Here we focus on EndoE, a multi-modular glycoside hydrolase secreted by Enterococcus faecalis, one of the leading causes of healthcare-associated infections. We provide X-ray crystal structures of EndoE, which show an architecture composed of four domains, including GH18 and GH20 glycoside hydrolases connected by two consecutive three α-helical bundles. We determine that the GH20 domain is an exo-β-1,2-N-acetylglucosaminidase, whereas the GH18 domain is an endo-β-1,4-N-acetylglucosaminidase that exclusively processes the central core of complex-type or high-mannose-type N-glycans. Both glycoside hydrolase domains act in a concerted manner to process diverse N-glycans on glycoproteins, including therapeutic IgG antibodies.

EndoE-GH20 crystallized in the P 1 2 1 1 space group with one molecule in the asymmetric unit and diffracted to a maximum resolution of 1.4 Å. The quality of the electron density maps allowed us to trace residues 489–835. The GH20 domain adopts the conserved (β/α)8-barrel topology with an overall size of 55 × 50 × 39 Å. A long and open groove, including a deep pocket, runs parallel to the protein surface and contains the active site. This groove is located at the center of the (β/α)8-barrel and surrounded by the loops connecting β1-α1 (loop 1; residues 499–505, pink), β2-β3 (loop 2; residues 530–541, brown), β5-α4 (loop 3; residues 598–603, orange), β6-α6 (loop 4; residues 660–670, light green), β7-β8 (loop 5; residues 706–724, blue), β8-α7 (loop 6; residues 729–740, green), β9-α8 (loop 7; residues 754–771, light blue), and β10-α9 (loop 8; residues 804–813, red). In a first step, D661 stabilizes the reaction intermediate and orients the acetamido oxygen for nucleophilic attack on the anomeric carbon to form an oxazolium ion intermediate. In addition, E662 acts as an acid protonating the glycosidic bond. Structural comparison of GH20 domain of EndoE with LNBase showed that the conformation and length of loops 1 and 8 in EndoE-GH20 could block the entrance of an extra carbohydrate moiety linked to GlcNAc (-1), confirming the exo-activity of this domain. The GH20 domain of EndoE cannot accommodate bisecting CT N-glycans due to the presence of bulky and hydrophobic residues in loop 7 that block the access of the additional β(1,4)-GlcNAc to the binding site, as in the case of the GH20A domain of StrH.

> GGSGQTQPLKSVFSIDAGRKYFSVEQLEELVAKASQNGYTDVQLILGNDGLRFILDDMSVNVNGKKYNHNRVSKAIQRGNNAYYNDPNGNALTQKEMDRLLAFAKARNINIIPVINSPGHMDALLVAMEKLAIKNPAFDGSKRTVDLGNQKAVNFTKAIISKYVAYFSAHSEIFNFGGDEYANDVDTGGWAKLQSSGRYKDFVAYANDLAKIIKDAGMQPMSFNDGIYYNSDDSFGTFDPEIIISYWTAGWSGYDVAKPEYFVQKGHKIFNTNDAWYWVAGNVDSGIYQYDDALANMSKKAFTDVPAGSPNLPIIGSIQCVWYDDPRRDYDFERIYTLMDTFSENYREYMVVKNH;> GAGAA5-HYDROXYMETHYLENE-6-HYDROFOLIC ACID | C20 H23 N7 O7 | 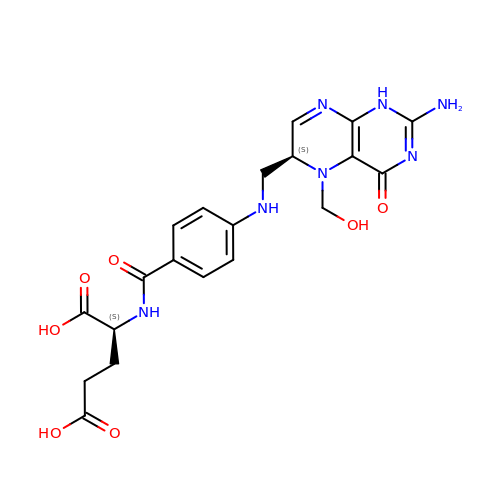IIEPLRAFVCMHQF-STQMWFEESA-N>MAHHHHHHMKDLLEIDGARLWRSLADMARIGATPRGGVRRLALTDDDRRGRDLFAQWCRDAGMTVSVDAVGNLFARRDGADAQAAPVLIGSHLDTQPEGGRFDGVYGVLAGLEVVRTLNDAGIVTDKPLEIVSWTNEEGARFAPAMLGSAVFTGALPLDDALARQDAEGITLGAALDACGCRGTRAPGGAVDAYFEAHIEQGPVLEANGTTIGIVTGGQAIRWLDVRVTGVAAHAGTTPMPYRKDAYFASAQMALELERIVAGHAPRGLATIGQAGIRNASRNTIAGDVTFTVDLRHHDDAQVDAMERALRDACARVAAARGVQVAIDTCWRSPATPFDRGCVELVARAAEAFGYTNERIVSGAGHDAILLARRVPTAMVFIPCVDGLSHNEAEDALPDDVTRGTNVLLNAVL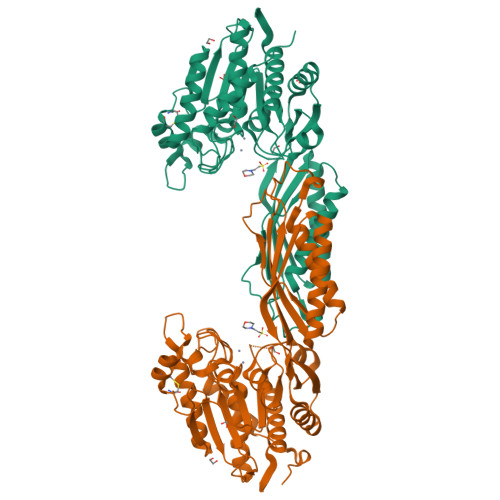ARAGVATRVAAAAAAHDA[2x]> MACRCTQLQDTIDEVATQFYSSIH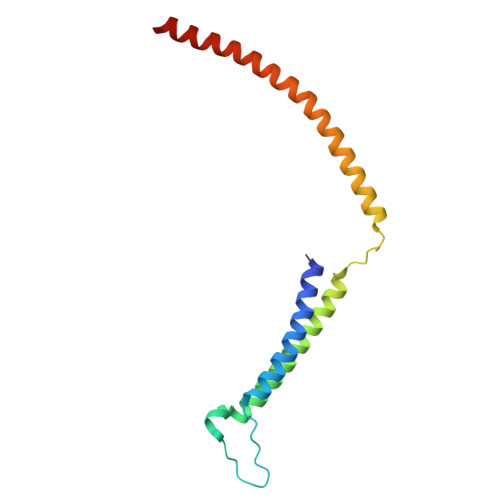YLSSHHDFVPLPGQEKVSDSKVNPISAEELQFAQRDLAKDLVTKFMQIDTLINQLPGISTAPKHQLEKIKKLQNSIEEKQLERKSLESENEDLKLQLAKRIETFGRLSCVLFQP>[2x]MRGSHHHHHHGMASELALPVGKLSESLFEPGKTDIRPSLVHGQISDIKTKPAYLRNVIKDGDLVNMKHKNLMKCAMDTPYIDKDMIDEAYQLTKSVWLKGMRDELKKVLTYEEAICGSEVSEYISSINRSSSPGYPWIKDRTKGTKGKQGWFGSEGEYILNEDVRLAVQQRIQAAREGKRLPVMWVDTLKDERRPIEKVNQLKTRVFSNGPMDFSIAFRMYYLGFIAHLMENRITNEVSIGTNVYSQDWSKTVRKLTKFGNKVIAGDFSTFDGSLNVCIMEKFADLANEFYDDGKENNLIRHVLLMDVYNSVHICNDSVYMMTHSQPSGNPATTPLNCFINSMGLRMCFAICAKNAGIKMTMKDFGKHVSM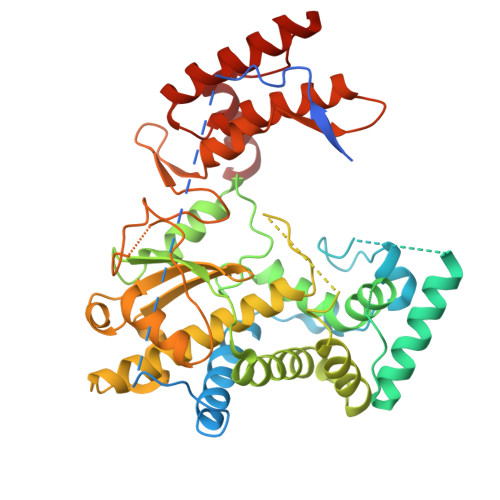VSYGDDNVINFSDEVCEWYNMETIAKAFETLGFTYTDELKGVNGEVPKWRSIKDVQYLKRKFRYDEQRKVWEAPLCMDTILEMPNWCRGGLDIQEGTKLNCENAIMELSMHEESVFDTWSKIIDRAYANATGDHLDINTYRGYAQERFLEYYM> MSMLVVVTENVPPRLRGRLAIWLLEVRAGVYVGDVSAKIREMIWEQIAGLAEEGNVVMAWATNTETGFEFQTFGLNRRTPVDLDGLR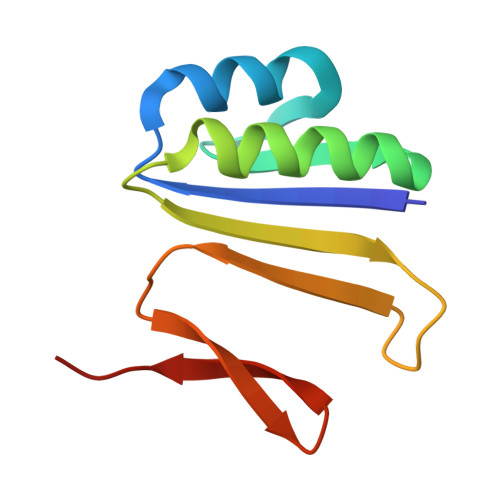LVSFLPVG> DKKTEETTNIEDRIETTVVGVTIINSQG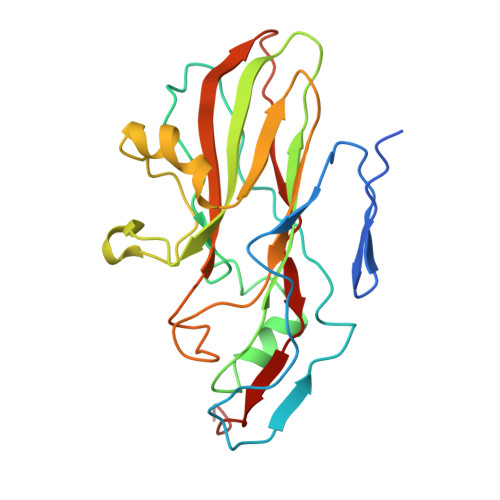SVGTTYCYSKPDGRPPSTVSDPVTRLGPTLSRHYTFKVGEWPHSQSHGHAWICPLPSDKLKKMGSFHEVVKAHHLVKNGWDVVVQVNASFAHSGALCVAAVPEYEHTHEKALKWSELEEPAYTYQQLSVFPHQLLNLRTNSSVHLVMPYIGPGPTTNLTLHNPWTIVILILSELTGPGQTVPVTMSVAPIDAMVNGPLPNPE>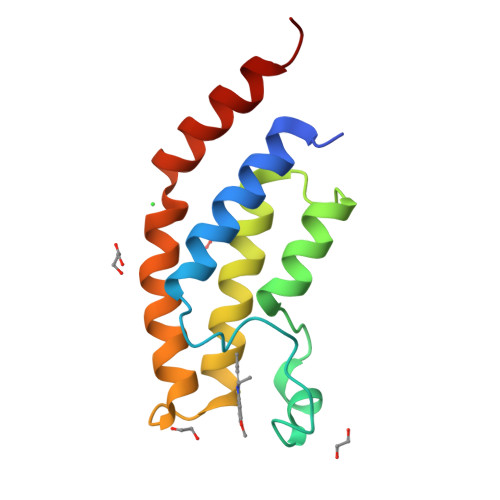[4x]ESEVEQTPLQEALNQLMRQLQRKDPSAFFSFPVTDFIAPGYSMIIKHPMDFSTMKEKIKNNDYQSIEELKDNFKLMCTNAMIYNKPETIYYKAAKKLLHSGMKILSQERIQSLKQSIDFMADL> MAFAHFVLIHTICHGAWIWHKLKPLLEALGHKVTALDLAASGVDPRQIEEIGSFDEYSEPLLTFLEALPPGEKVILVGESCGGLNIAIAADKYCEKIAAAVFHNSVLPDTEHCPSYVVDKLMEVFPDWKDTTY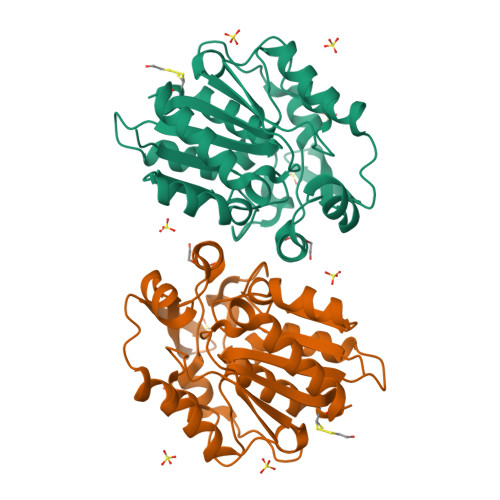FTYTKDGKEITGLKLGFTLLRENLYTLCGPEEYELAKMLTRKGSLFQNILAKRPFFTKEGYGSIKKIYVWTDQDEIFLPEFQLWQIENYKPDKVYKVEGGDHKLQLTKTKEIAEILQEVADTYN>[2x]SQFEQPRTIQEEGSDPFDLKPDSISKAITDRLYHISDGKILGFIPNQYLDPESSLIEDDFLLIYVYTYELPLLSAVFVPEYNCYEIAITNVAKFFSKIGVRSYPHSIKNSLLELKELIDNNRYDITIYKKEFTIGAAKSSKWALKDVVLRSALPTPKEVTFTENKFPLVRVSNIVPSASSRYYTVIGLAVTVKYTGGKTLVLSFTDFTANPKVNYGYDSFLGSFQERIPENEHVHALIYLNRVESLNEKLQSIIKMGL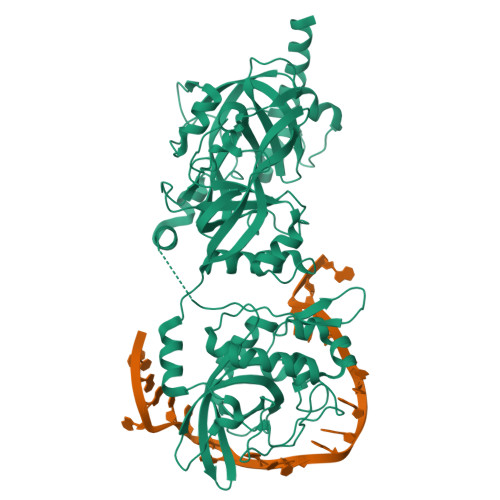MECADKGNSNITHRSIIFKFTVKCQLFQGKLNTVILDADPITPTTPVTTEEYKLLKPLRNKIFKRMPSEVIQLYTLTMSRFLPISKNRMSENPQLLQEQAFYDSAGSSEDPKDDSIAKLENQLKREGVDKIEEDAATRPIELFGTRNPKTVDIIDIKNNVQMDHKDIKVTAKILSIFDNGNNVTIYLTRSGMVGTQCTIENPFEELLKVQIWGRQNLTLFFGNPNYSYKREELTACIGSIVDFTLIPRVLRVNEYLYIKIWCPIYATLESLLIHSRLEYDNDTLKYENLSDID>[3x]MLQAACPESWIGFQRKCFYFSDDTKNWTS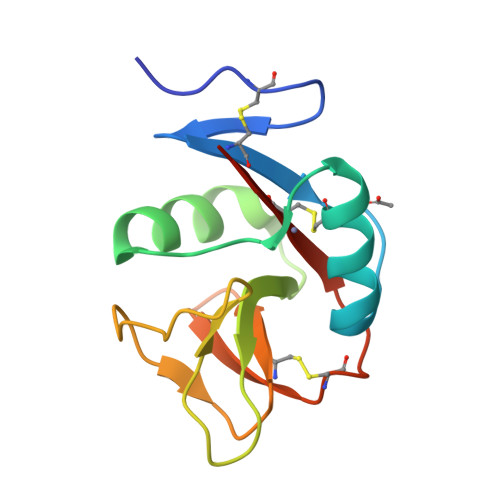SQRFCDSQDADLAQVESFQELNFLLRYKGPSDHWIGLSREQGQPWKWINGTEWTRQFPILGAGECAYLNDKGASSARCYTERKWICSKSDIHV1-[3-(4-chlorophenyl)propyl]imidazole | C12 H13 Cl N2 | 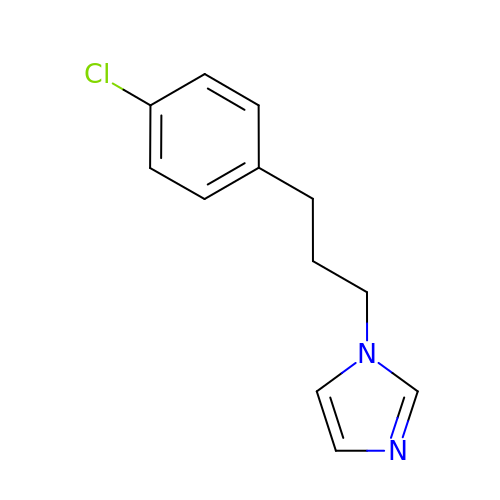CLJJKXWBLJQDDT-UHFFFAOYSA-N> QKPQRPRRPASPISTIQPKANFDAQQFAGTW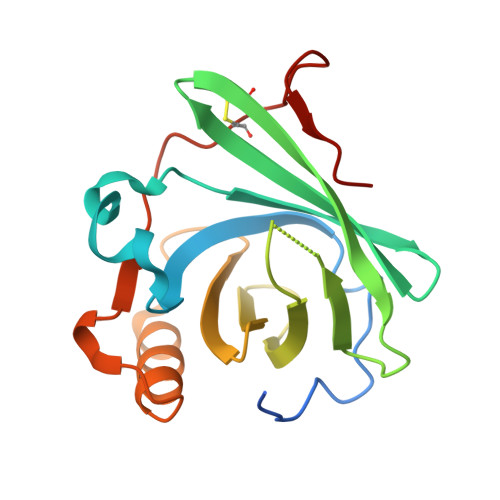LLVAVGSACRFLQEQGHRAEATTLHVAPQGTAMAVSTFRKLDGICWQVRQLYGDTGVLGRFLLQARDARGAVHVVVAETDYQSFAVLYLERAGQLSVKLYARSLPVSDSVLSGFEQRVQEAHLTEDQIFYFPKYGFCEAADQFHVLDEVRR>[4x]MVNVAVIGAAGGIGQSLSLLLLRELPFGSTLSLYDVVGAPGVAADLSHIDRAGITVKHAAGKLPPVPRDPALTELAEGVDVFVIVAGVPRKPGMTRDDLFNVNAGIVMDLVLTCASVSPNACFCIVTNPVNSTTPIAAQTLRKIGVYNKNKLLGVSLLDGLRATRFINNARHPLVVPYVPVVGGHSDVTIVPLYSQIPGPLPDESTLKEIRKRVQVAGTEVVKAKAGRGSATLSMAEAGARFTMHVVKALMGLDTPMVYAYVDTDGEHECPFLAMPVVLGKNGIERRLPIGPITTVEKEMLEEAVGVVKKNIAKGETFARSKL;>MDCSTGAAIGQQFAKDAFHMHGGVGVGPTGNSEHDVLMNEMMMVQTPTGPAGEWTHQFAAYQGQQQQQQQQHPQELAMRHQQNDAFMLRQQQEMEEAFCTFCTTHPHSHAHSHQPQGLVGPAMMGPQIMPPMMFGPGTGGFMMGAPPMMPYASMKFAGDAAMAAANNTNMTQGAT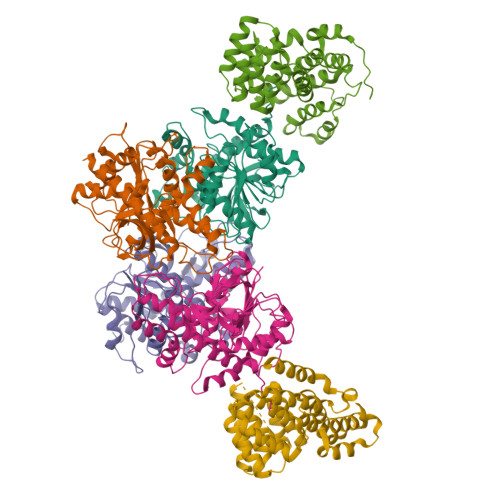ATSTTSVQQELQQQSSDNGWVEKLRDAEWAQDYSDAQVFTLEGQSEQTMEEHAKNSEFYQFMDKIRSKELLIDEETGQLVQGPGPDPDAPEDAEYLKEWAAAEGLNMPPGFFEHMMQRPQGNNEQAEGRLFDGSNDALMDDGALDNAADVEEWVREYAEAQEQLQRVQNETNYPFEPNNPYMYHDKPMEEGIAMLQLANMAEAALAFEAVCQKEPENVEAWRRLGTTQAENEKDCLAIIALNHARMLDPKDIAVHAALAVSHTNEHNVGAALQSLRSWLLSQPQYEHLGLVDLREVAADEGLDEVPEENYFFAAPSEYRDCCTLLYAAVEMNPNDPQLHASLGVLHNLSHRFDEAAKNFRRAVELRPDDAHMWNKLGATLANGNRPQEALEAYNRALDINPGYVRVMYNMAVSYSNMAQYPLAAKHITRAIALQAGGTNPQGEGSRIATRGLWDLLRMTLNLMDRSDLVEASWQQDLTPFLREFGLEEMAV[2x]> TSASED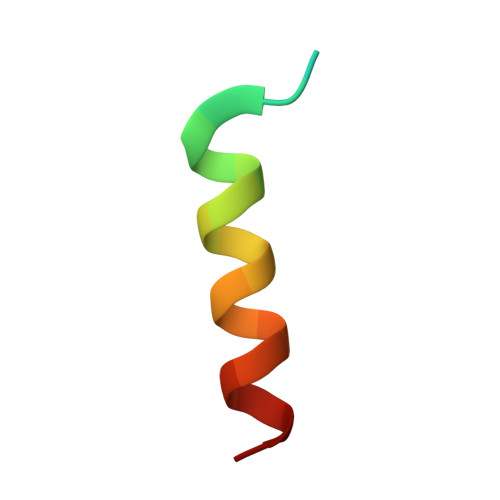IDFDDLSRRFEELKKKT> ADVPAGVQLADKQTLVRNNGSEVQSLDPHKIEGVPESNVSRDLFEGLLISDVEGHPSPGVAEKWENKDFKVWTFHLRENAKWSDGTPVTAHDFVYSWQRLAD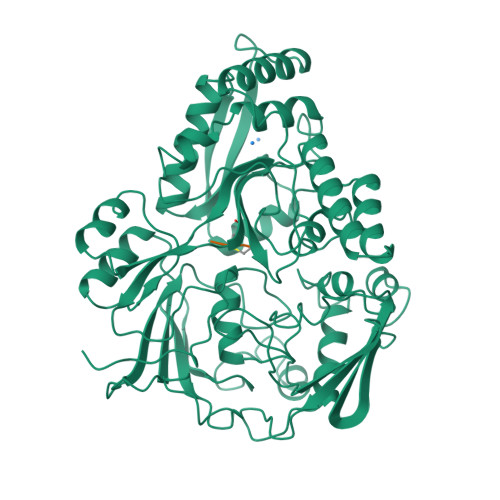PNTASPYASYLQYGHIANIDDIIAGKKPATDLGVKALDDHTFEVTLSEPVPYFYKLLVHPSVSPVPKSAVEKFGDKWTQPANIVTNGAYKLKNWVVNERIVLERNPQYWDNAKTVINQVTYLPISSEVTDVNRYRSGEIDMTYNNMPIELFQKLKKEIPNEVRVDPYLCTYYYEINNQKAPFNDVRVRTALKLALDRDIIVNKVKNQGDLPAYSYTPPYTDGAKLVEPEWFKWSQQKRNEEAKKLLAEAGFTADKPLTFDLLYNTSDLHKKLAIAVASIWKKNLGVNVNLENQEWKTFLDTRHQGTFDVARAGWCADYNEPTSFLNTMLSDSSNNTAHYKSPAFDKLIADTLKVADDTQRSELYAKAEQQLDKDSAIVPVYYYVNARLVKPWVGGYTGKDPLDNIYVKNLYIIKH;> VKPG1-METHOXY-2-[2-(2-METHOXY-ETHOXY]-ETHANE | C8 H18 O4 | 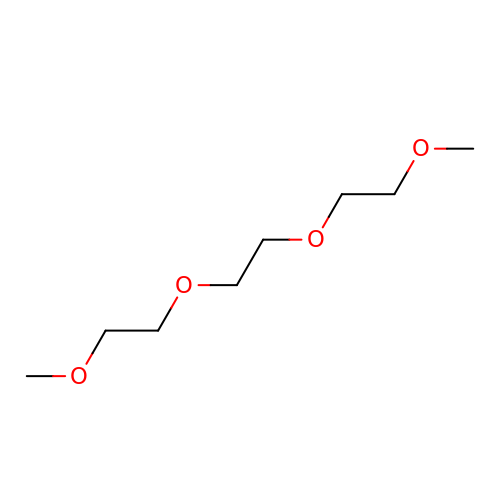YFNKIDBQEZZDLK-UHFFFAOYSA-N>[2x]ETGTPMMPPVGVQASILSHDTIRITWADNSLPKHQKITDSRYYTVRWKTNIPANTKYKNANATTLSYLVTGLKPNTLYEFSVMVTKGRRSSTWSMTAHGATFELVPTSPPKDVTVVSKEGKPRTIIVNWQPPSEANGKITGYIIYYSTDVNAEIHDWVIEPVVGNRLTHQIQELTLDTPYYFKIQARNSKGMGPMSEAVQFRTPKADSSDKMPNDQALGSAGKGSRLPDLGSDYKPPMSGSNSPHGSPTSPLDSNGTKHHHHHH;>ETGQPAQCRIQKCTTDFVSLTSHLNSAVDGFDSEFCKALRAYAGCTQRTSKACRGNLVYHSAVLGISDLMSQRNCSKDGPTSSTNPEVTHDPCNYHSHAGAREHRRGDQNPPSYLFCGLFGD[2x];>PHLRTFKDNFQTCKVEGAWPLIDNNYLSVQVTNVPVVPGSSATATNKITIIFKAHHGCTDQKVYQAVTDDLPAAFVDGTTSGGDSDAKSLRIVERESGHYVEMHA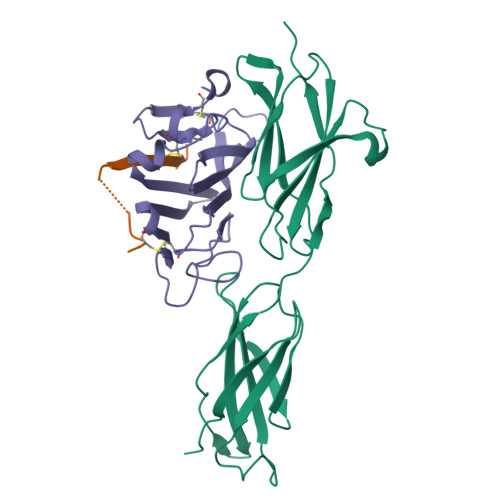RYIGTTVFVRQVGRYLTLAIRMPEDLAMSYEESQDLQLCVNGCPLSERIDDGQGQVSAILGHSLPRTSLVQAWPGYTLETANTQCHEKMPVKDIYFQSCVFDLLTTGDANFTAAAHSALEDVEALHPRKERWHIFPSGTKHHHHHH[2x]> VPPGEDSKDVAAPHRQPLTSSERIDKQIRYILDGISALRKETCNKSNLCESSKEALAENNLNLPKMAEKDGCFQSGFNEETCLVKIITGLLEFEVYLEYLQNRFESSEEQARAVQMSTKVLIQFLQKKAKNLDAITTPDPTTNASLLTKLQAQNQWLQDMTTH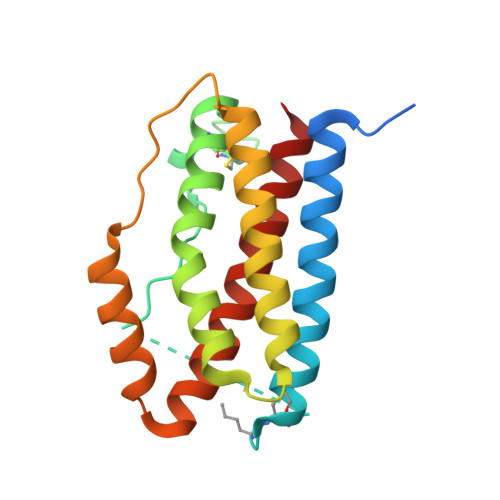LILRSFKEFLQSSLRALRQM>TYTTRQIGAKNTLEYKVYIEKDGKPVS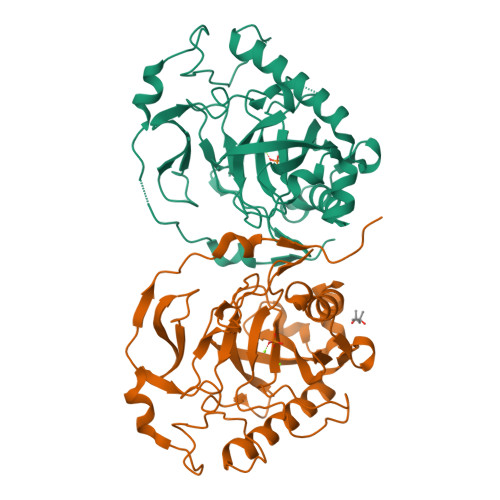AFHDIPLYADKENNIFNMVVDIPRWTNAKLEITKEETLNPIIQDTKKGKLRFVRNCFPHHGYIHNYGAFPQTWEDPNVSHPETKAVGDNDPIDVLEIGETIAYTGQVKQVKALGIMALLDEGETDWKVIAIDINDPLAPKLNDIEDVEKYFPGLLRATNEWFRIYKIPDGKPENQFAFSGEAKNKKYALDIIKETHDSWKQLIAGKSSDSKGIDLTNVTLPDTPTYSKAASDAIPPASLKADAPIDKSIDKWFFISGSV[2x]>XQARSDIEKLKEAIRDTNKAVQSVQSSIGNLIVAIKSVQDYVNKEIVPSIARX[3x];>[3x]XV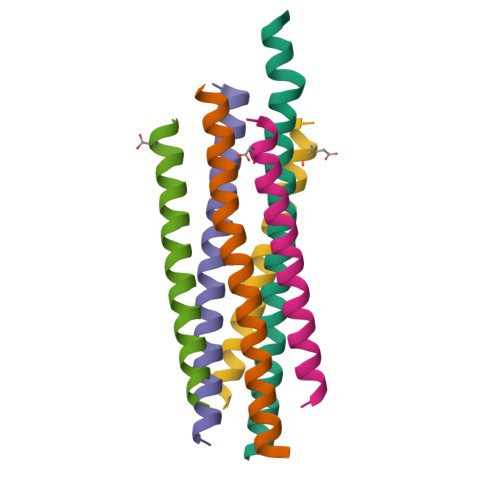ALDPIDISIVLNKIKSQLEESKEWIRRSNKILDSIX> MIIKPAGDSAFLISFGDEIS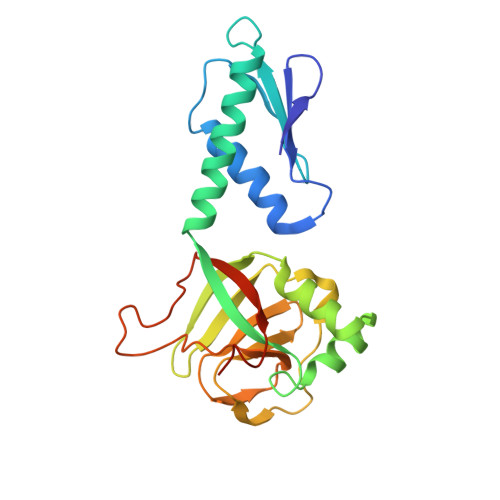EEINDRVHSLAKAIEKESPEWLVELVPAYSSLLVIYDPLKASYEEVESYLKRISAREVERIKGKTIEIPVAYGGEFGPDIEFVAQYNGLSVDDVIEIHSKPLYRVYFLGFLPGFAYLGGMDERIATPRLEKPRLKVPAGSVGIAGKQTGWYAIESPGGWRIIGRIPLRTFNPGKVPPSIVLPGDYVKFVPIDEKEFWEIYGREWE>[2x]MRLLPSSCAGALSLLCSLAIAAPTELKARDLSSFIASERAIALQGALNNIGPDGSAVPGAGAGFVVASPSKANPDYFYTWSRDSALTLKMIIDEFILGNTTLQTIIEQYIHAQAVLQTVSNPSGTFLPDGVGLGEPKFMVDGTRFNGPWGRPQRDGPALRAIALMTYSNWLIKNGQFAEAKTKIWPIIANDLSYVGQYWNQSGFDLWEETYASSFFTIQNQHRALVEGAQLAHDLGVTCTGCDQAPEVLCFLQSFWNGKYIVSNINVNNGRTGLDGNSILGAISTFDIDAYCDSPTLQPCHSQSLANFKVLTDTFRNLYTINAGIPEGQGVAVGRYAEDVYMGGNPWYLITTAAAEFLYDAVAQWKARHVLTVDETSLAFFKDIYPEVTVREYKSGNANSPFAQIMDAVTAYADSYVAIAEKYIPSNGSLSEQFNRDTGTPLSAIDLTWSYAAFITMSQRRAGQYPSSWGSRNALPPPTTC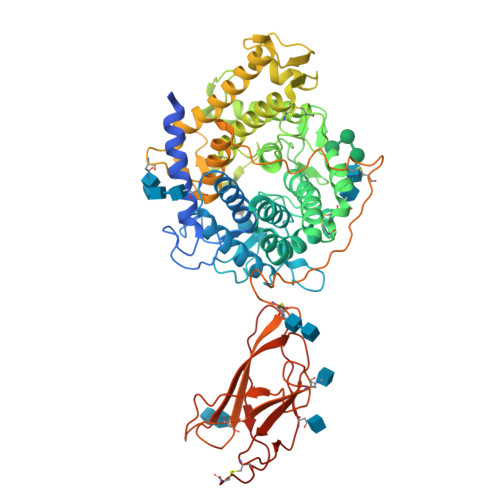SASSTPGIYTPATAAGAPNVTSSCQVSITFNINATTYYGENLYVIGNSSDLGAWNIADAYPLSASAYTQDRPLWSAAIPLNAGEVISYQYVRQEDCDQPYIYETVNRTLTVPACGGAAVTTDDAWMGPVGSSGNC>MKKNGKSQNQPLDFTQYAKNMRKDLSNQDICLEDGALNHSYFLTKKGQYWTPLNQKALQRGIELFGVGNWKEINYDEFSGKANIVELELRTCMILGINDITEYYGKKISEEEQEEIKKSNIAKGKKENKLKDNIYQKLQQMQ[2x];>DDYLDRLPKSKKGLQGLLQDIEKRILHYKQLFFKEQNEIANGKRSMVPDNSIPICSDVTKLNFQALIDAQMRHAGKMFDVIMMDPPWQLSSSQPSRGVAIAYDSLSDEKIQNMPIQSLQQDGFIFVWAINAKYRVTIKMIENWGYKLVDEITWVK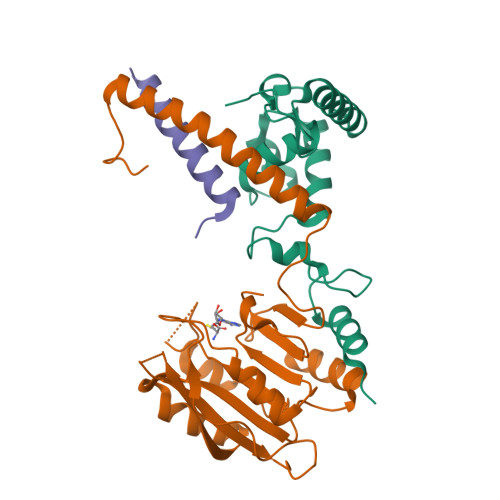KTVNGKIAKGHGFYLQHAKESCLIGVKGDVDNGRFKKNIASDVIFSERRGQSQKPEEIYQYINQLCPNGNYLEIFARRNNLHDNWVSIGNEL[2x];>MSLKKGKFQHNQSKSLWNYTLSPGWREEEVKILKSALQLFGIGKWKKIMESGCLPGKSIGQIYMQTQRLLGQQSLGDFMGLQIDLEAVFNQNMKKQDVLRKNNCIINTGDNPTKEERKRRIEQNRKIYGLSAKQIAEIKLPKVKKHAPQYMTLEDIENEKFTNLEILTHLYNLKAEIVRRLAEQGETIAQPSIIKSLNNLNHNLEQNQNSNSSTETKVTLEQSGKKKYKVLAIEETELQNGPIATNSQKKSINGKRKNNRKINSDSEGNEEDISLEDIDSQESEINSEEIVEDDEEDEQIEEPSKIKKR[2x]>SDRNVMNSDMKKNIVQWNSRYSYNQLKNKDSLIMFLVEIFRSLFVSNCIDKNIDNVLLSIEEMFIDHYYNPQHSRLKYLIDDVGIFFTKLPITKAFHTYNKKYRITKRLYAPPTFNEVRHILNLAQILSLEEGLDLLTFDANETLYPDGHDFNDEVLASYISCLLKKMNIAIVTAASYNNDAEKYQKRLENLLKYFSKHNIKDGSYKNFYVMGGESNYLFKCNEEATLYSVPENEWRHYKKFVDYDTVQEILNISEKCLEKVIKDFGLCAQIQRKEKSIGLVPNKIPSLNIKNEQKNY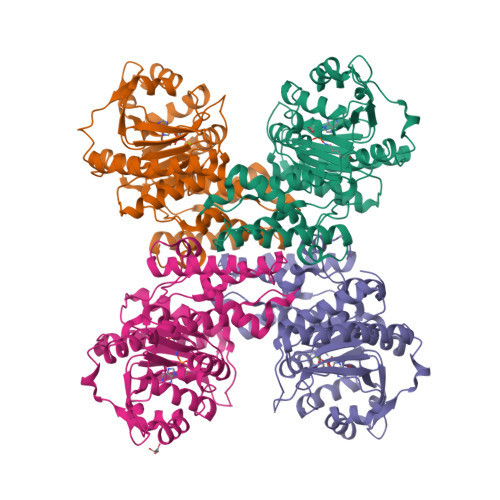MIKYEVLEEAVIRIKKEIIKNKITAPYCAFNGGQDLWVDVGNKAEGLLILQKLLKIQKKKCCHIGDQFLHSGNDFPTRFCSLTLWVSNPQETKACLKSIMHLNIKSFIPEVLYENQ[8x]>[4x]QTKKAAIVELLKQLELGLVPYDDIKQLIRRELARRLQWGYKPTYEEQIAEIQNLTHSLRQMKIATEVETLDSQLYEIPIEFLKIMNGSNLKGSCCYFKEDSTTLDEAEIAMLDLYCERAQIQDGQSVLDLGCGQGALTLHVAQKYKNCRVTAVTNSVSQKEYIEEESRRRNLLNVEVKLADITTHEMAETYDRILVIELFEHMKNYELLLRKISEWISKDGLLFL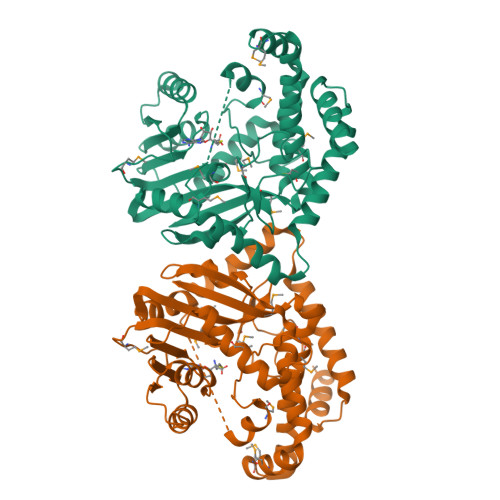EHICHKTFAYHYEPLDDDDWFTEYVFPAGTMIIPSASFFLYFQDDVSVVNHWTLSGKHFSRTNEEWLKRLDANLDVIKPMFETLMGNEEEAVKLINYWRGFCLSGMEMFGYNNGEEWMASHVLFKK> MSQSVSERTRIKSDRYESGVIPYAKMGYWDAAYSVKDTDVLALFRITPQPGVDPVEAAAAVAGESSTATWTVVWTDLLTAC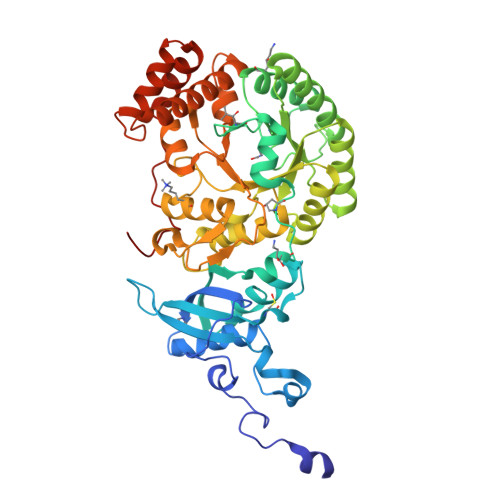ERYRAKAYRVDPVPNSTDVYFAFIAYECDLFEEASLSNLTASIIGNVFGFKAISALRLEDMRIPHSYLKTFQGPATGIIVERERLNKYGTPLLGATVKPKLGLSGKNYGRVVYEGLKGGLDFLKDDENINSQPFMRWRERFLNCLEGINRAAAATGEVKGSYLNITAATMEEVYKRAEYAKAIGSVVVMIDLVMGYTAIQSIAYWARENDMLLHLHRAGNSTYARQKNHGINFRVICKWMRMSGVDHIHAGTVVGKLEGDPLMIKGFYDVLRLTELEVNLPFGIFFEMDWASLRRCMPVASGGIHCGQMHQLIHYLGDDVVLQFGGGTIGHPDGIQAGATANRVALEAMVLARNEGADYFNNQVGPQILRDAAKTCGPLQTALDLWKDISFNYTSTDTADFAETATANR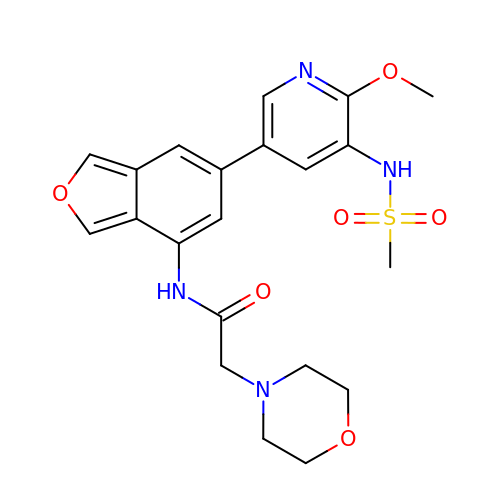N-[6-(5-methanesulfonamido-6-methoxypyridin-3-yl)-1,3-dihydro-2-benzofuran-4-yl]-2-(morpholin-4-yl)acetamide | C21 H24 N4 O6 S | BZDMXCRKVCKVEV-UHFFFAOYSA-N> METDTLLLWVLLLWVPGSTGDAAQPARRANGSEWSYTNILTGPETWHEHYKNMCSGYYQSPIDLKT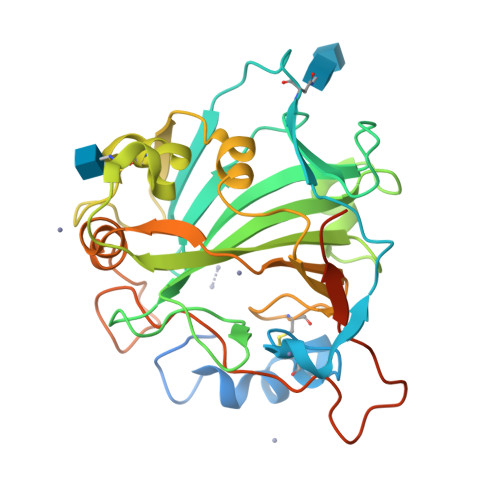DISTLDLKLKTVIIYRNTSSTETTTIQNNGHSAEVKFPRNTWFISFDGILDYKYEIIQMHFHWGNTDDRGSEHTIDGFRFPLEGHIVSFRRQMYSSPSEAIGRPGGLAVLGIMHQIVESIKYEQTAFKAYNNFSGVLNSQFVPPNNSTIDDINLALLLSLLNPSRYFRYLGSLTTPPCTENVLWTVFIDPVLITREQINLFRNLPYGSNEKQTRMGDNFRPIQLLNPIDTLASRTLYRATARGGPEQKLISEEDLNSAVDHHHHHH>[2x]GSHMASKPIEDYGKGKGRIEPMYIPDNTFYNADDFLVPPHCKPYIDKILLPGGLVKDRVEKLAYDIHRTYFGEELHIICILKGS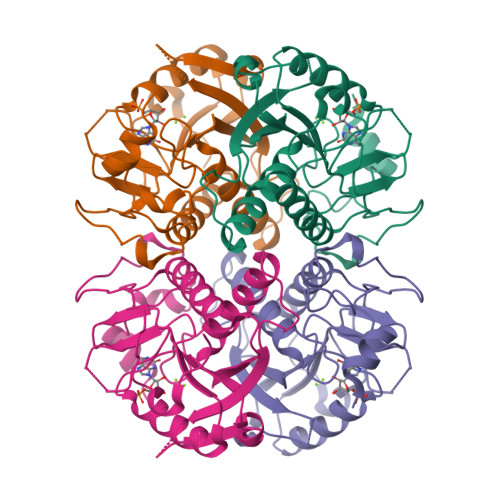RGFFNLLIDYLATIQKYSGRESSVPPFFEHYVRLKSYQNDNSTGQLTVLSDDLSIFRDKHVLIVEDIVATGFTLTEFGERLKAVGPKSMRIATLVEKRTDRSNSLKGDFVGFSIEDVWIVGCCYDFNEMFRDFDHVAVLSDAARKKFEK>[12x]AMGTTVLPPLEDTDGLWAALTEAAASVEKLLATLPEHGARSSAERAEIAAAHDAARALRVRFLDTHADAVYDRLTDHRRVHLRLAELVEAAATAFPGLVPTQQQLAVERSLPQAAKEGHEIDQGIFLRAVLRSPLAGPHLLDAMLRPTPRALELL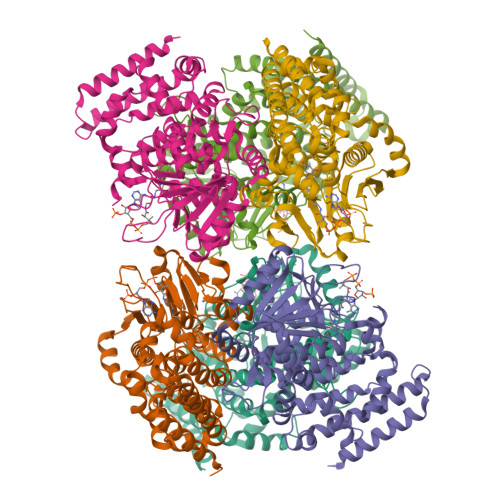PEFVRTGEVEMEAVHLERRDGVARLTMCRDDRLNAEDGQQVDDMETAVDLALLDPGVRVGLLRGGVMSHPRYRGKRVFSAGINLKYLSQGGISLVDFLMRRELGYIHKLVRGVLTNDDRPGWWHSPRIEKPWVAAVDGFAIGGGAQLLLVFDRVLASSDAYFSLPAAKEGIIPGAANLRLGRFAGPRVSRQVILEGRRIWAKEPEARLLVDEVVEPDELDAAIERSLTRLDGDAVLANRRMLNLADESPDGFRAYMAEFALMQALRLYGHDVIDKVGRFGGRPPA>GSFVEMVDNLRGK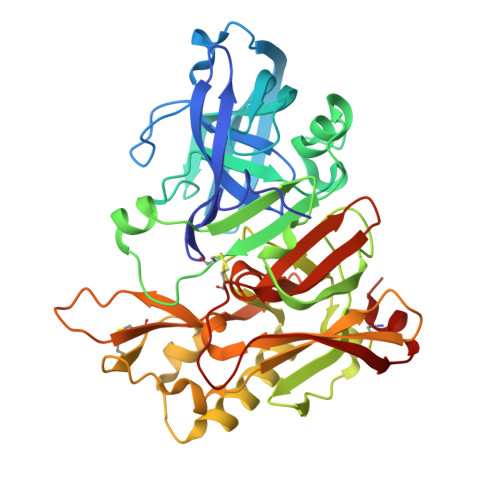SGQGYYVEMTVGSPPQTLNILVDTGSSNFAVGAAPHPFLHRYYQRQLSSTYRDLRKGVYVPYTQGKWEGELGTDLVSIPHGPNVTVRANIAAITESDKFFINGSNWEGILGLAYAEIARPDDSLEPFFDSLVKQTHVPNLFSLQLCGAGFPLNQSEVLASVGGSMIIGGIDHSLYTGSLWYTPIRREWYYEVIIVRVEINGQDLKMDCKEYNYDKSIVDSGTTNLRLPKKVFEAAVKSIKAASSTEKFPDGFWLGEQLVCWQAGTTPWNIFPVISLYLMGEVTNQSFRITILPQQYLRPVEDVATSQDDCYKFAISQSSTGTVMGAVIMEGFYVVFDRARKRIGFAVSACHVHDEFRTAAVEGPFVTLDMEDCGYN[4x];> KTEEISEVNXVAEF> VVGGEDAKPGQFPWQVVLNGKVDAFCGGSIVNEKWIVTAAHCVETGVKITVVAGEHNIEETEHTEQKRNVIRIIPHHNYNAAINKYNHDIALLELDEPLVLNSYVTPICIADKEYTNIFLKFGSGYVSGWGRVFHKGRSALVL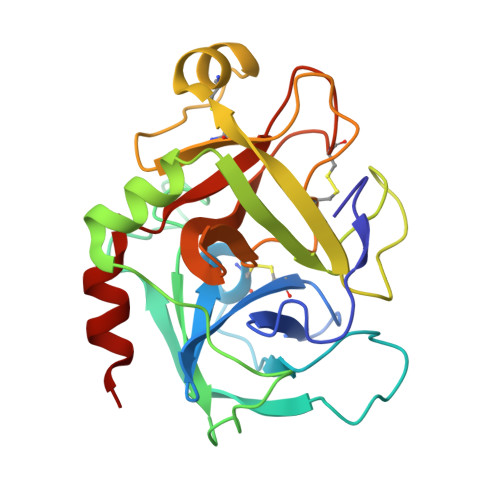QYLRVPLVDRATCLRSTKFTIYNNMFCAGFHEGGRDSCQGDSGGPHVTEVEGTSFLTGIISWGEECAMKGKYGIYTKVSRYVNWIKEKTKLT> GSHAWDTAN;> SDQNVDSRDPVQLNLLYVQARDDILNGSHPVSFDKACEFAGYQCQIQFGP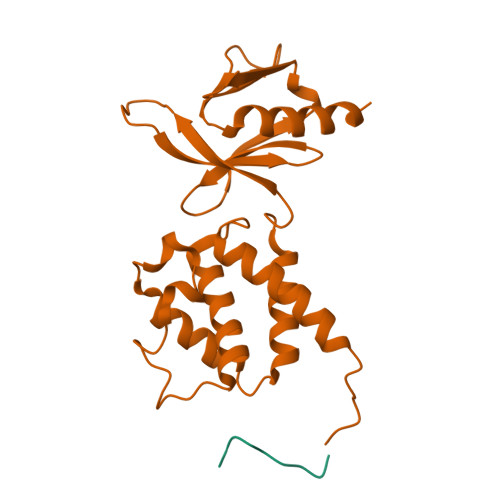HNEQKHKPGFLELKDFLPKEYIKQKGERKIFMAHKNCGNMSEIEAKVRYVKLARSLKTYGVSFFLVKEKMKGKNKLVPRLLGITKECVMRVDEKTKEVIQEWSLTNIKRWAASPKSFTLDFGDYQDGYYSVQTTEGEQIAQLIAGYIDIIL> GGGGKAWPTHVVCSDSGLEVLYQSCDPLQDFGFSVEKCSKQLKSNINIRFGIILREDIKELFL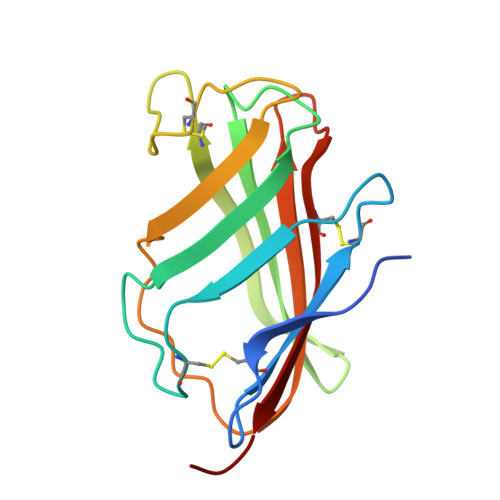DLALMSQGSSVLNFSYPICEAALPKFSFCGRRKGEQIYYAGPVNNPEFTIPQGEYQVLLELYTEKRSTVACANATIMCSEF>MVQVNLKAAKKQKFTPEEDEMLKRAVAQHGSDW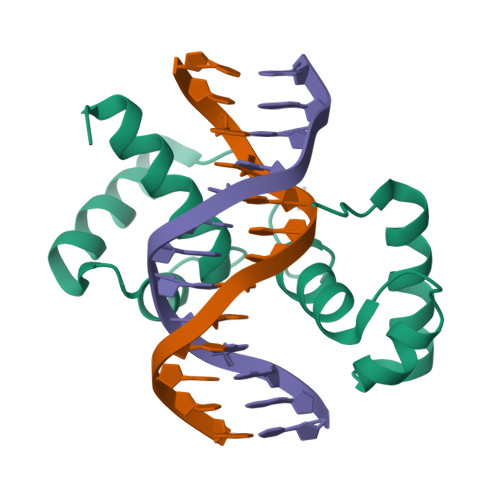KMIAATFPNRNARQCRDRWKNYLAPSISHTPWTAEEDALLVQKIQEYGRQWAIIAKFFPGRTDIHIKNRWVTISNKLGIPQTQQMLEHHHHHH[2x]>MVSKLSQLQTELMAALLESGLSKEALIQALGE[2x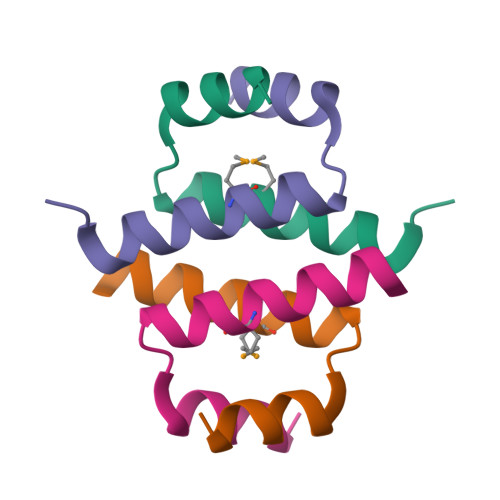]>MSAAPGLLHQELSCPLCLQLFDAPVTAECGHSFCRACLGRVAGEPAADGTVLCPCCQAPTRPQALSTNLQLARLVEGLAQVPQGHCEEHLDPLSIYCEQDRALVCGVCASLGSHRGHRLLPAAEAHARLKTQLPQQKLQLQEACMRKEKSVAVLEHQLVEVEETVRQFRGAVGEQLGKMRVFLAALEGSLDREAERVRGEAGVALRRELGSLNSYLEQLRQMEKVLEEVADKPQTEFLMKYCLVTSRLQKILAESPPPARLDIQLPIISDDFKFQVWRKMFRALMPALEELTFDPSSAHPSLVVSSSGRRVECSEQKAPPAGEDPRQFDKAVAVVAHQQLSEGEHYWEVDVGDKPRWALGVIAAEAPRRGRLHAVPSQGLWLLGLREGKILEAHVEAKEPRALRSPERRPTRIGLYLSFGDGVLSFYDASDADALVPLFAFHERLPRPVYPFFDVCWHDKGKNAQPLLLVGPEGAEA[2x]

Human TRIM72, a tripartite motif family protein primarily found in striated muscle, consists of four domains: the RING domain, B-box domain, coiled-coil domain, and SPRY domain. Tripartite Motif Protein 72 (TRIM72, also named MG53) mediates membrane damage repair through membrane fusion and exocytosis. During injury, TRIM72 molecules form intermolecular disulfide bonds in response to the oxidative environment and TRIM72 oligomers are proposed to connect vesicles to the plasma membrane and promote membrane fusion in conjunction with other partners like dysferlin and caveolin.

After extensive optimization, we managed to obtain relatively well-diffracting crystals and determined the structure of the TRIM72 dimer at 3.0 Å. In the structure, we observed electron density for TRIM72 B-box, coiled-coil, and SPRY domains (BCC-SPRY), but the RING domain is not observed despite the fact that we used full-length protein for crystallization. The overall shape of TRIM72 BCC-SPRY dimer is similar to that of a clothes hanger. Residues (122–230) form a long α2 helix which in turn forms an antiparallel dimer with the α2′ helix from the other molecule. The short α4 helix (residues 270 to 283) again forms an antiparallel dimer with α4′ helix from the other protomer. Both ends of the coiled-coil domain are covered by a B-box domain. The two globular SPRY domains sit above the coiled-coil domain at the midpoint, with one on each side. In the TRIM72 structure, the α4 dimer packs tightly with the center region of the long α2 dimer to form an X-shaped junction with three layers of hydrophobic interactions. The SPRY domain is not flexibly linked to the coiled-coil domain as generally believed, instead, the SPRY domain of TRIM72 formed extensive interactions with the α4 helices. Zinc atom 1 (ZN1) is coordinated by C86, H89, C105, and C108; zinc atom 2 (ZN2) is coordinated by C97, D100, H114, and H117, the use of an aspartate instead of Cys/His for ZN2 coordination is similar to what has been observed for TRIM5α B2-box. One direct result of TRIM72 B-box dimerization is that the C242 residues from two TRIM72 molecules are brought to a close distance of 30 Å, possibly facilitating disulfide bond formation.> SEDDLTKVLNYTKQRQTEPNPEYYGVAKKKNIIKIHLESFQTFLINKKVNGKEVTPFLNKLSSGKEQFTYFPNFFHQTGQGKASDSEFTMDNSLYGLPQGSAFSLKGDNTYQSLPAILDQKQGYKSDVMHGDYKTFWNRDQVYKHFGIDKFYDATYYDMSDKNVVNLGLKDKIFFKDSANYQAKMKSPFYSHLITLTNHYPFTLDEKDATIEKSNTGDATVDGYIQTARYLDEALEEYINDLKKKGLYDNSVIMIYGDHYGISENHNNAMEKLLGEKITPAKFTDLNRTGFWIKIPGKSGGINNEYAGQVDVMPTILHLAGIDTKNYLMFGTDLFSKGHNQVVPFRNGDFITKDYKYVNGKIYSNKNNELITTQP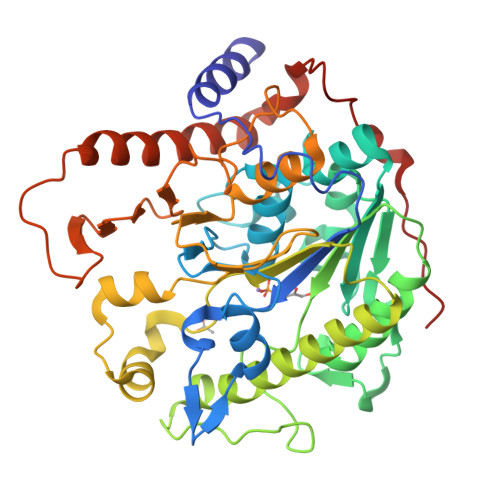ADFEKNKKQVEKDLEMSDNVLNGDLFRFYKNPDFKKVNPSKYKYETGPK> HLRAYHQKIDSNLDELSMGLGRLKDIALGMQTEIEEQDDILDRLTTKVDKLDVNIKSTERKV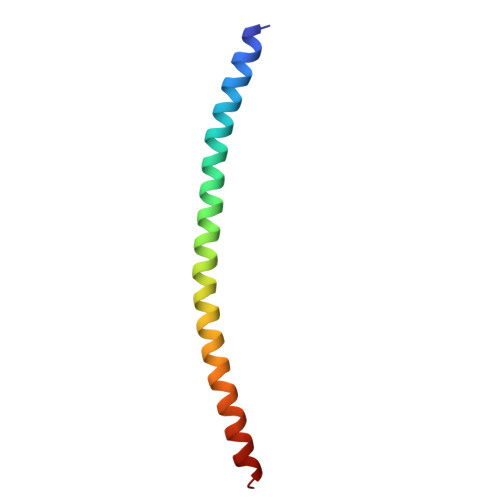RQL> MALLSKKVMNFAYGMGAAVVIVGALFKITHFEIGPLTGTVMLSIGLLTEALIFALSAFEPVEDELDWTLVYPELANGQARKKEAKAETATDAQGLLSQKLDAMLKEAKVDGELMASLGNSIKNFEGAAKAISPTVDSIAGQKKYAEEMSMAAAQMESLNSLYKVQL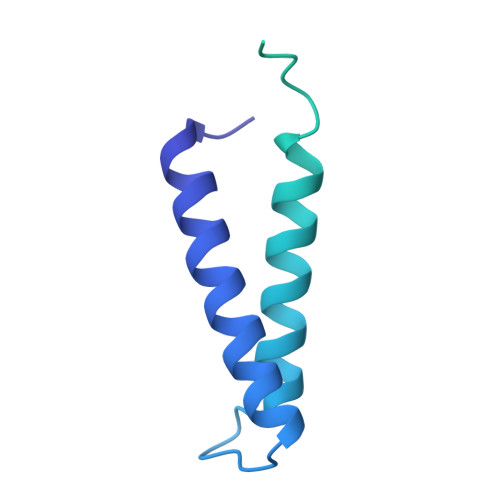ESASRNAQANSEIAENAAKLKEQMASMTANIASLNSVYGGMLSAMSNKG>[3x]MASGSMHLRPIATPYPVKEWLQPKRYKAHLMGTTYVYDFPELFRQASSSQWKNFSADVKLTDDFFISNELIEDEN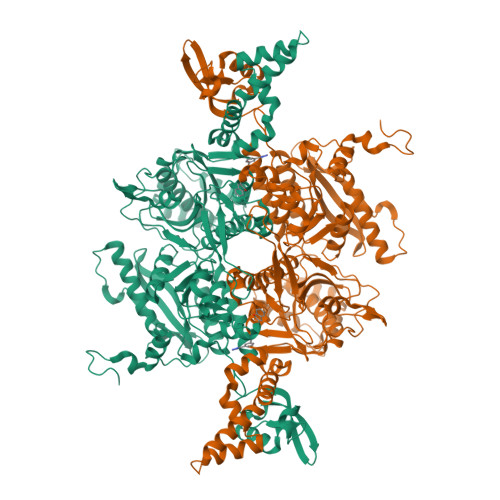GELTEVEREPGANAIGMVAFKITVKTPEYPRGRQFVVVANDITFKIGSFGPQEDEFFNKVTEYARKRGIPRIYLAANSGARIGMAEEIVPLFQVAWNDAANPDKGFQYLYLTSEGMETLKKFDKENSVLTERTVINGEERFVIKTIIGSEDGLGVECLRGSGLIAGATSRAYHDIFTITLVTCRSVGIGAYLVRLGQRAIQVEGQPIILTGASALNKVLGREVYTSNLQLGGTQIMYNNGVSHLTAVDDLAGVEKIVEWMSYVPAKRNMPVPILETKDTWDRPVDFTPTNDETYDVRWMIEGRETESGFEYGLFDKGSFFETLSGWAKGVVVGRARLGGIPLGVIGVETRTVENLIPADPANPNSAETLIQQAGQVWFPNSAFKTAQAINDFNNGEQLPMMILANWRGFSGGQRDMFNEVLKYGSFIVDALVDYKQPIIIYIPPTGELRGGSWVVVDPTINADQMEMYADVNARAGVLEPEGTVEIKFRREKLLDTMNRLDDKYRELRSQLSNKSLAPEVHQQISKQLADRERELLPIYGQISLQFADLHDRSSRMVAKGVISKELEWTEARRFFFWRLRRRLNEEYLIKRLSHQVGEASRLEKIARIRSWYPASVDHEDDRQVATWIEENYKTLDDKLKGLKLESFAQDLAKKIRSDHDNAIDGLSEVIKMLSTDDKEKLLKTLKLEHHHHHH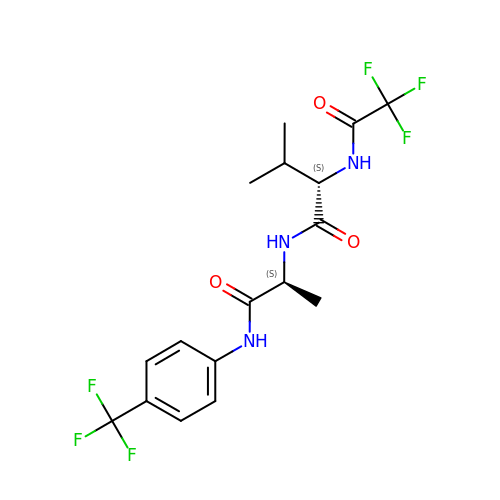N-(trifluoroacetyl)-L-valyl-N-[4-(trifluoromethyl)phenyl]-L-alaninamide | C17 H19 F6 N3 O3 | XAJBYSREBDCYAJ-CABZTGNLSA-N>[2x]MTMSPCPLLLVFVLGLVVIPPTLAQNERYEKFLRQHYDAKPQGRDDRYCESMMKERKLTSPCKDVNTFIHGTKKNIRAIC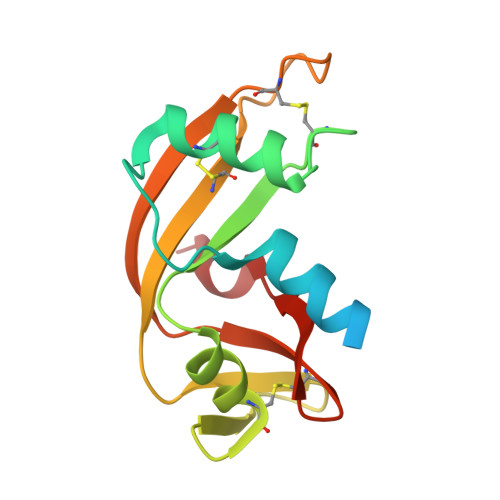GKKGSPYGENFRISNSPFQITTCTHSRGSPWPPCGYRAFKDFRYIVIACEDGWPVHFDESFISP> MTHGAVKTYGIRLRVWGDYACFTRPEMKVERVSYDVMPPSAARGILEAIHWKPAIRWIVDRIHVLRPIVFDNVRRNEVSSKIPKPNPATAMRDRKPLYFLVDDGSNRQQRAATLLRNVDYVIEAHFELTDKAGAEDNAGKHLDIFRRRARAGQSFQQPCLGCREFPASFELLEGDVPLSCYAGEKRDLGYMLLDIDFERDMTPLFFKAVMEDGVITPP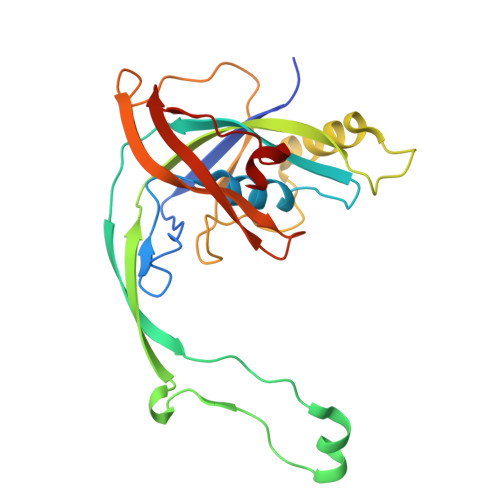SRTSPEVRA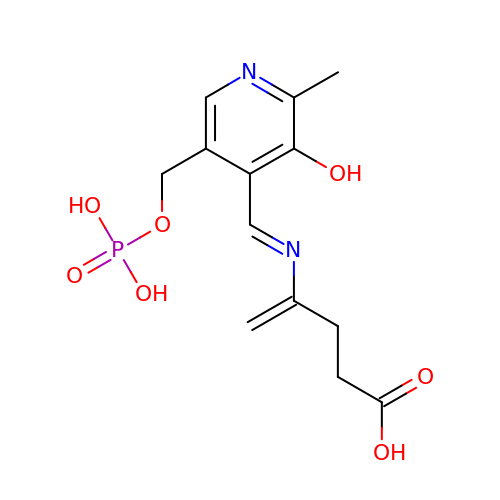4-[(E)-({3-hydroxy-2-methyl-5-[(phosphonooxy)methyl]pyridin-4-yl}methylidene)amino]pent-4-enoic acid | C13 H17 N2 O7 P | HRCALJQKZAULQS-MKMNVTDBSA-N> MVVLSVPAEVTVILLDIEGTTTPIAFVKDILFPYIEENVKEYLQTHWEEEECQQDVSLLRKQAEE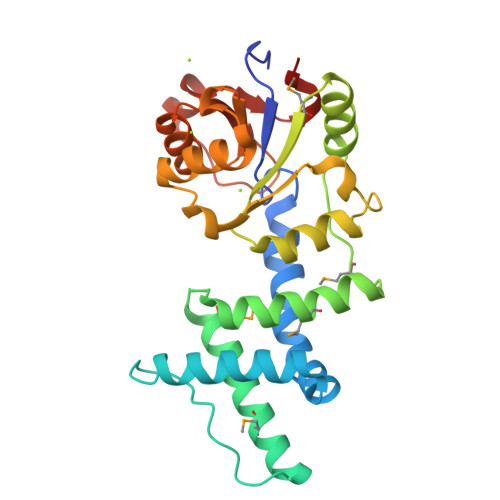DAHLDGAVPIPAASGNGVDDLQQMIQAVVDNVCWQMSLDRKTTALKQLQGHMWRAAFTAGRMKAEFFADVVPAVRKWREAGMKVYIYSSGSVEAQKLLFGHSTEGDILELVDGHFDTKIGHKVESESYRKIADSIGCSTNNILFLTDVTREASAAEEADVHVAVVVRPGNAGLTDDEKTYYSLITSFSELYLPSST>SNAMNSQLTLRALERGDLRFIHNLNNNRNIMSYWFEEPYESFDELEELYNKHIHDNAERRFVVEDAQKNLIGLVELIEINYIHRSAEFQIIIAPEHQGKGFARTLINRALDYSFTILNLHKIYLHVAVENPKAVHLYEECGFVEEGHLVEEFFINGRYQDVKRMYILQSK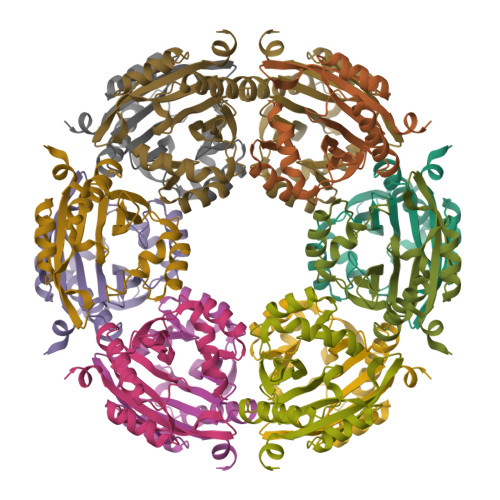YLNRSE[3x]>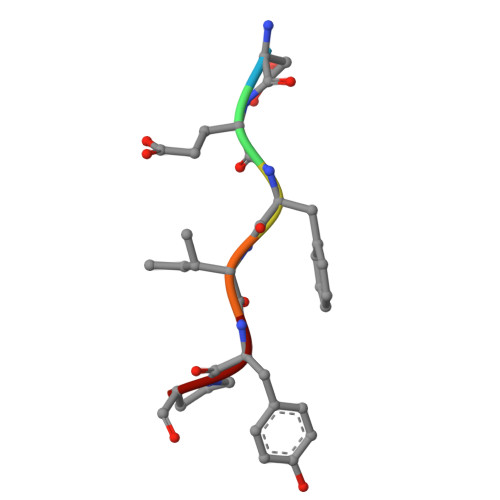 DEFIYP>GRRGVLMTLLQQSAMTLPLWIGKPGDKPPPLCGAIPASGDYVARPGDKVAARVKAVDGDEQWILAEVVSYSHATNKYEVDDIDEEGKERHTLSRRRVIPLPQWKANPETDPEALFQKEQLVLALYPQTTCFYRALIHAPPQRPQDDYSVLFED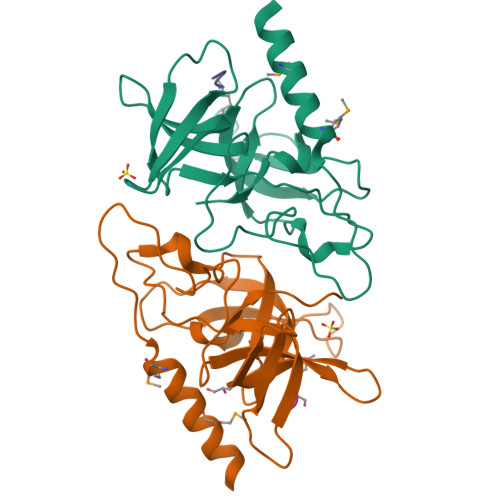TSYADGYSPPLNVAQRYVVACKEPKKK[2x];>[2x]AATKQTAR During replication, herpesviral capsids are translocated from the nucleus into the cytoplasm by an unusual mechanism, termed nuclear egress, that involves capsid budding at the inner nuclear membrane. Capsid budding at the INM requires the viral nuclear egress complex (NEC), a heterodimer of two conserved viral proteins: UL31, a soluble nuclear phosphoprotein, and UL34, which contains a single C-terminal transmembrane (TM) helix that anchors the NEC in the INM. Here, we report the crystal structure of the NEC from Epstein-Barr virus (EBV), a prototypical gammaherpesvirus. Here, we show that the purified, recombinant EBV NEC vesiculates synthetic lipid membranes in vitro and forms membrane-bound coats, which suggests that the intrinsic membrane budding ability is a conserved property of the NECs across Herpesviridae.

For crystallization, we designed a construct EBV NEC195Δ65 composed of residues 1–195 of BFRF1 and residues 66–318 of BFLF2, which is similar to those of previously crystallized NEC homologs. This construct lacks the membrane-proximal regions (MPRs) in both BFRF1 and BFLF2 as well as the TM anchor of BFRF1. The structure was refined to 3.97 Å resolution (Rwork = 27.0%, Rfree = 30.8%). Like its counterparts in alpha- and betaherpesviruses, the EBV NEC resembles an elongated cylinder that is composed of the globular BFRF1 pedestal topped with the globular C-terminal domain of BFLF2 and the N-terminal two-helix “hook” of BFLF2 that wraps around the BFRF1 pedestal. The conserved CCCH-type Zn-binding site, formed by three cysteines and one histidine, is located at the base of the globular domain. Importantly, EBV NEC crystals contain five independent, structurally distinct heterodimers in the asymmetric unit. The structural differences among the 5 EBV NEC heterodimers, notably within BFLF2 and at the BFLF2/BFRF1 interface, for the first time experimentally demonstrate conformational dynamics within the EBV NEC. BFLF2 interacts with BFRF1 at two interfaces, the so-called “primary” or hook-in-groove interface that involves the BFLF2 hook, and the “secondary” or globular interface, which involves the globular domain of BFLF2. Across the five EBV NEC heterodimers, the globular domains of BFLF2 adopt distinct orientations relative to BFRF1 where they are either more or less tilted towards the BFRF1/hook module, as measured by the angles between D10BFRF1/P98BFRF1/D287BFLF2. We attribute the differences in tilt across the EBV NEC heterodimers to the differences in the interactions at the globular domain interface, specifically, the presence or the absence of the distal hydrogen bond between T158BFRF1 and E250BFLF2.

>GPLGSMASPEERLLDELNNVIVSFLCDSGSLEVERCSGAHVFSRGSSQPLCTVKLRHGQIYHLEFVYKFLAFKLKNCNYPSSPVFVISNNGLATTLRCFLHEPSGLRSGQSGPCLGLSTDVDLPKNSIIMLGQDDFIKFKSPLVFPAELDLLKSMVVCRAYITEHRTTMQFLVFQAANAQKASRVMDMISDMSQQLSRSG[5x];>[5x]GPGSRSICSRHTRHGVDRSHFSLRDFFRGISANFELGKDFLREMNTPIHVSEAVFLPLSLCTLSPGRCLRLSPFGHSLTLGSHCEICINRSQVHVPQEFSSTQLSFFNNVHKIIPNKTFYVSLLSSSPSAVKAGLSQPSLLYAYLVTGHFCGTICPIFSTNGKGRLIMHLLLQGTSLHIPETCLKLLCENIGPTYELAVDLVGDAFCIKVSPRDTVYEKAVNVDEDAIYEAIKDLECGDELRLQIINYTQLILENKQ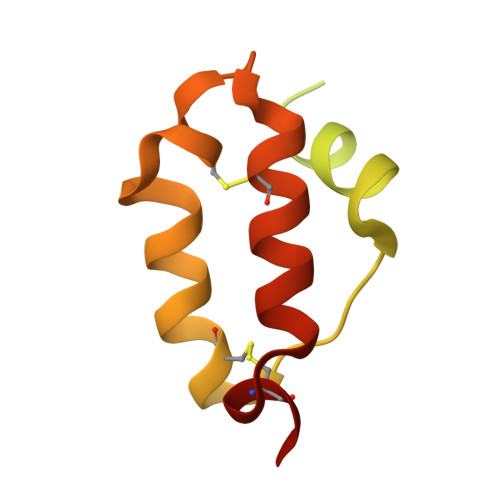> GAEPREPADGQALLRLVVELVQELRKHHSAEHKGLQLLGRDYALGRAEAAGLGPSPEQRVEIVPRDLRMKDKFLKHLTGPLYFSPKCSKHFHRLYHNTRDCTIPAYYKRCARLLTRLAVSPVCMEDKQ> X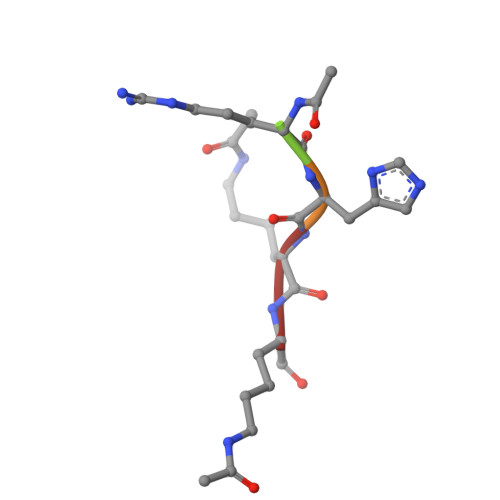RHKK>[2x]MAETRVIVVGNEKGGAGKSTIAVHLVTALLYGGAKVAVIDLDLRQRTSARFFENRRAWLDNKKIELPEPLALNLSDNDVALAERPEEEQVAGFEAAFARAMAECDFILIDTPGGDSAITRMAHGRADLVVTPMNDSFVDFDMLGTVDPVTLELTKPSLYSLTVWEGRKQRALSGQRQAMDWVVLRNRLATTEARNRKRLEDRLNALAKRVGFRIGPGLRDRVIYRELFPFGLTIADLSPQVRPVPVSLQHLAARQELRALMHSLGLSAYSGETMLAAQAVDKLAAALEHHHHHH

Protein gradients play a central role in the spatial organization of cells, but the mechanisms of their formation are incompletely understood. This study analyzes the determinants responsible for establishing bipolar gradients of the ATPase MipZ, a key regulator of division site placement in Caulobacter crescentus. MipZ dynamically interacts with the polar ParB-parS complexes, forming a subcellular gradient with concentration maxima at the tips of the cell and a minimum at the cell center. It inhibits polymerization of the tubulin homolog FtsZ into the so-called Z ring, a structure that forms the basis of the bacterial divison apparatus (Erickson et al., 2010). MipZ belongs to the Mrp/MinD family of P loop ATPases, a heterogeneous group of proteins that act as nucleotide-dependent molecular switches (Leipe et al., 2002).

The two independent structures show excellent agreement with a root-mean-square deviation (rmsd) of 0.44 Å. Superimposition of the structures reveals that MipZ, Soj and MinD share significant similarity in the region constituting the nucleotide-binding site, with an rmsd of 2.4 Å across the 176 α-carbons forming the backbone of the conserved core. However, MipZ differs from its family relatives in the arrangement of several conserved loops. In addition, it displays a number of unique features, including a marked extension of helix 2 and a large loop between helices 9 and 10 (helices 10/11 in Soj). Notably, helices 6 and 7 of MipZ correspond to a single helix in both Soj and MinD (helix 8 in Soj). At the junction of these two helices, MipZ exhibits an unusual structural motif, consisting of a large loop that is stabilized by a short antiparallel β sheet (S6/S7). Together, these distinct characteristics are consistent with a clear evolutionary separation of MipZ from its two relatives. MipZ has no C-terminal amphipathic helix, as used for membrane attachment of MinD, and lacks the conserved DNA-binding domain characteristic of plasmid-encoded ParA proteins (Gerdes et al., 2010). Interaction analyses showed that MipZ monomers bind to ParB irrespective of their nucleotide state. Monomers are unable to interact with the nucleoid and, consequently, display high diffusional mobility, thereby rapidly returning to the polar ParB clusters.>HHHHHHHHENLYFQGDPTQFEERHLKFLQQLGKGNFGSVEMCRYDPLQDNTGEVVAVKKLQHSTEEHLRDFEREIEILKSLQHDNIVKYKGVCYSAGRRNLKLIMEYLPYGSLRDYLQKHKERIDHIKLLQYTSQICKGMEYLGTKRYIHRDLATRNILVENENRVKIGDFGLTKVLPQDKEYYKVKEPGESPIFWYAPESLTESKFSVASDVWSFGVVLYELFTYIEKSKSPPAEFMRMIGNDKQGQMIVFHLIELLKNN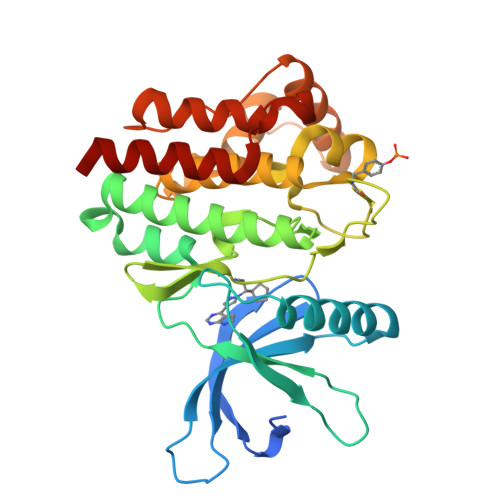GRLPRPDGCPDEIYMIMTECWNNNVNQRPSFRDLALRVDQIRDNMAG[4x]> TGQKLDDVDPLVATNFGKIRGIKKELNNEILGPVIQFLGVPYAAPPTGERRFQPPEPPSPWSDIRNATQFAPVCPQNIIDGRLPEVMLPVWFTNNLDVVSSYVQDQSEDCLYLNIYVPTEDDIRD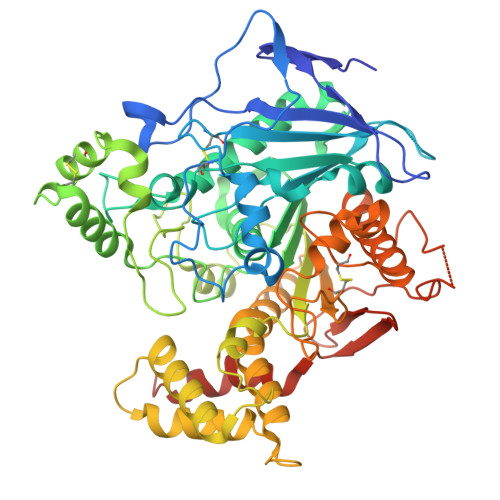SGGPKPVMVYIHGGSYMEGTGNLYDGSVLASYGNVIVITVNYRLGVLGFLSTGDQAAKGNYGLLDLIQALRWTSENIGFFGGDPLRITVFGSGAGGSCVNLLTLSHYSEGLFQRAIAQSGTALSSWAVSFQPAKYARMLATKVGCNVSDTVELVECLQKKPYKELVDQDIQPARYHIAFGPVIDGDVIPDDPQILMEQGEFLNYDIMLGVNQGEGLKFVENIVDSDDGISASDFDFAVSNFVDNLYGYPEGKDVLRETIKFMYTDWADRHNPETRRKTLLALFTDHQWVAPAVATADLHSNFGSPTYFYAFYHHCQTDQVPAWADAAHGDEVPYVLGIPMIGPTELFPCNFSKNDVMLSAVVMTYWTNFAKTGDPNQPVPQDTKFIHTKPNRFEEVAWTRYSQKDQLYLHIGLKPRVKEHYRANKVNLWLELVPHLHNLNDRTKHHHHHH>MSSVKISPLKDSEAFQSIKVGNNTLQTKIVYPPTTRFRALEDHTPSDLQLQYYGDRSTFPGTLLITEATFVSPQASGWEGAAPGIWTDKHAKAWKVITDKVHANGSFVSTQLIFLGRVADPAVMKTRGLNPVSASATYESDAAKEAAEAVGNPVRALTTQEVKDLVYEAYTNAAQKAMDAGFDYIELHAAHGYLLDQFLQPCTNQRTDEYGGSIENRARLILELIDHLSTIVGADKIGIRISPWATFQNMKAHKDTVHPLTTFSYLVHELQQRADKGQGIAYISVVE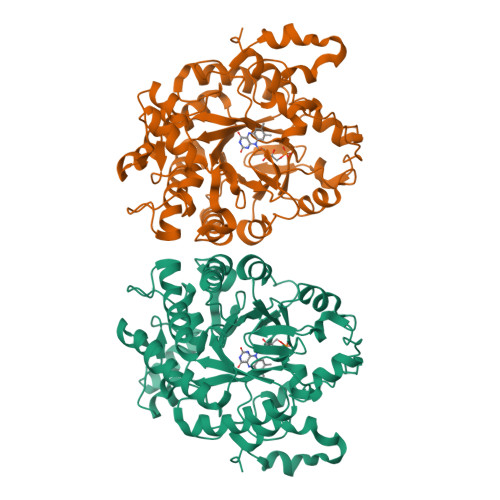PRVSGNVDVSEEDQAGDNEFVSKIWKGVILKAGNYSYDAPEFKTLKEDIADKRTLVGFSRYFTSNPNLVWKLRDGIDLVPYDRNTFYSDNNYGYNTFSMDSEEVDKELEIKRVPSAIEAL[6x]> XADVAGTSNRDFRGREQRLFNSEQYNYNSSLNGEVSVWVYAYYSDGSVLVINKNSQYKVGISETFKALKEYRKGQHNDSYDEYEVNQSIYYPNGGDARKFHSNAKPRAIQIIFSPSVNVRTIKMAKGNAVSVPDEYLQRSHPWEATGIKYRKIKRDGEIVGYSHYFELPHEYNSISLAVSGVHKNPSSYNVGSAHNVMDVFQSCDLALRFCNRYWAELELVNHYISPNAYPYLDINNHSYGVA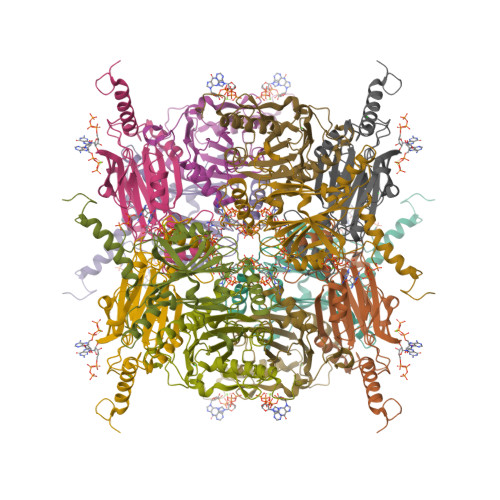LSNRQ> PNFSGNWKIIRSENFEELLKVLG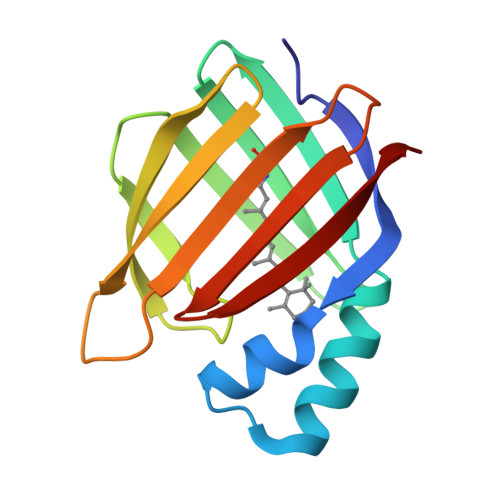VNVMLRKIAVAAASKQAVEIKQEGDTFYIKVSTTVYTTEINFKVGEEFEEQTVDGRPCKSLVKWESENKMVCEQKLLKGEGPKTSWTKELTNDGELILTMTADDVVCTQVFVRE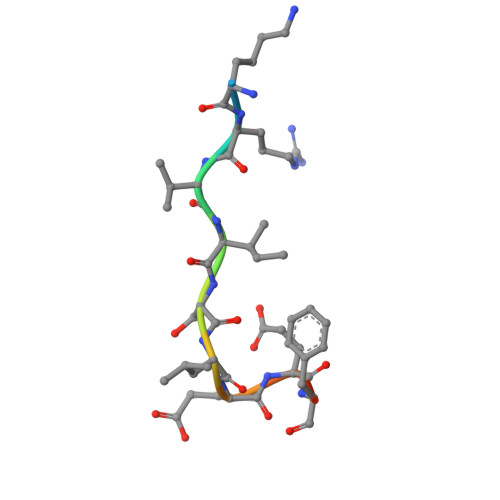> KKRVISLEEFFS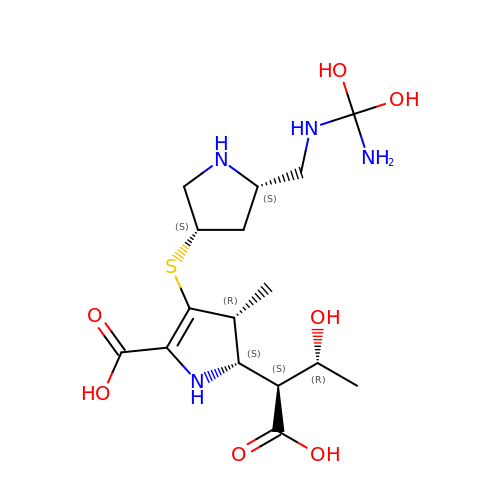(4R,5S)-3-{[(3S,5S)-5-({[amino(dihydroxy)methyl]amino}methyl)pyrrolidin-3-yl]sulfanyl}-5-[(1S,2R)-1-carboxy-2-hydroxypropyl]-4-methyl-4,5-dihydro-1H-pyrrole-2-carboxylic acid | C16 H28 N4 O7 S | VAWRCDOEVLBCMW-VFZPANTDSA-N> GG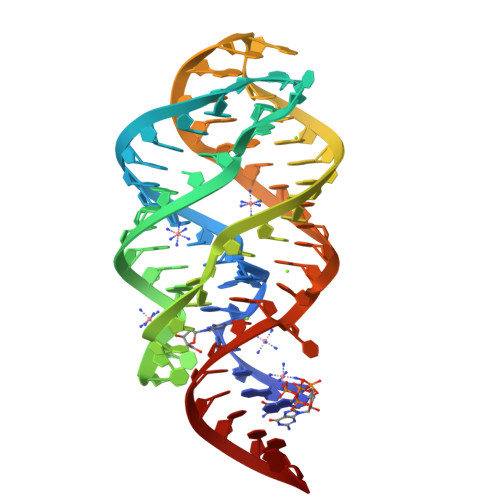GUGUAAUCUCCAAAAUAUGGUUGGGGAGCCUCCACCAGUGAACCGUAAAAUCGCUGUCACCACCCAG4-fluoro-2-{[4-(pyridin-4-yl)-1,3-thiazol-2-yl]amino}phenol | C14 H10 F 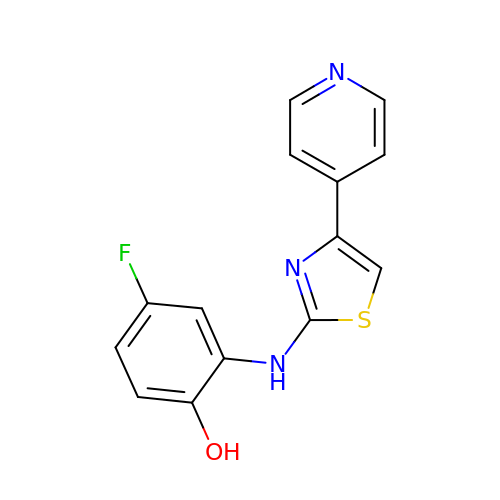N3 O S | RMWZRYBJQMKPMA-UHFFFAOYSA-N>[2x]MPREYEFAEKILFTEEEIRTRIKE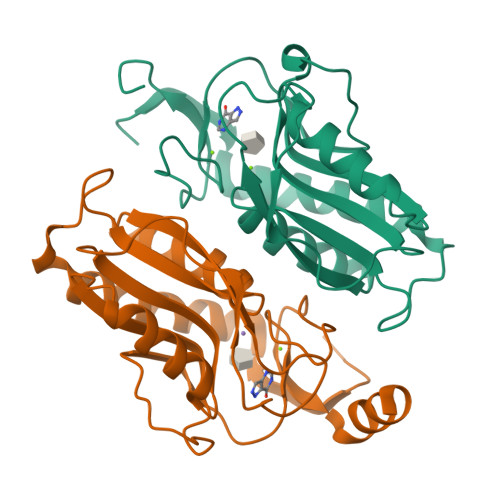VAKRIADDYKGKGLRPYVNPLVLISVLKGSFMFTADLCRALCDFNVPVRMEFICVSSYGEGLTSSGQVRMLLDTRHSIEGHHVLIVEDIVDTALTLNYLYHMYFTRRPASLKTVVLLDKREGRRVPFSADYVVANIPNAFVIGYGLDYDDTYRELRDIVVLRPEVYAEREAARQKKQRAIGSADTDRDAKREFHSKY>MIRVACVGITVMDRIYYVEGLPTESGKYVARNYTEVGGGPAATAAVAAARLGAQVDFIGRVGDDDTGNSLLAELESWGVNTRYTKRYNQAKSSQSAIMVDTKGERIIINYPSPDLLPDAEWLEEIDFSQWDVVLADVRWHDGAKKAFTLARQAGVMTVLDGDITPQDISELVALSDHAAFSEPGLARLTGVKEMASALKQAQTLTNGHVYVTQGSAGCDWLENGGRQHQPAFKVDVVDTTGAGDVFHGALAVALATSGDLAESVRFAS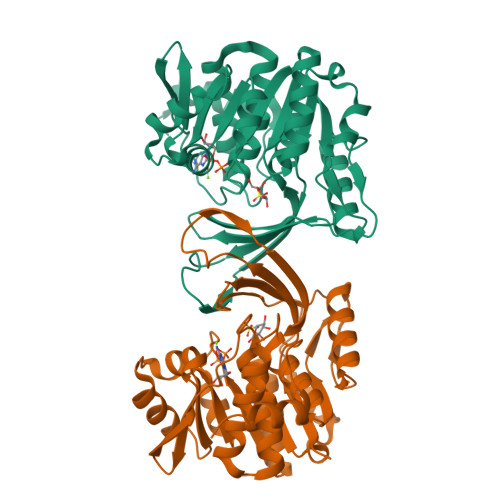GVAALKCTRPGGRAGIPDCDQTRSFLSLFVLEHHHHHH[2x]>ALFALSLPVLAGPAVTPSSQIETDLLPASLLQISETEAFSRYVILVDKEQRKLSVFERNGEQIQKITEYPADIGKMGGNKTKRDDHKTPEGIYFLQERLSQPKIPFSLYGALAFTTNYPNLFDKRENKTGSGIWLHAIPDSVPLTRGSRGCVVVRNDVIKKLADYIKLGETPILIFDHVNYVSKSEHDKRRQDLSRFVESWRQAWENQDIEKYQTFYDEGFKAP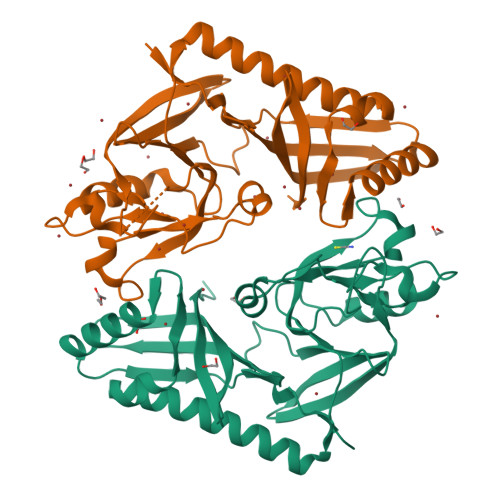GFNYKSWMSHKKNLKSKYEYIKVHLSQPYIVQHNDQLLVKTLQRYESDKHVDYGVKTIYALKSGDTYKIIREEWAPFSQQEVAAAIARENSMTASSQKTQ[2x]>[2x]SNIEV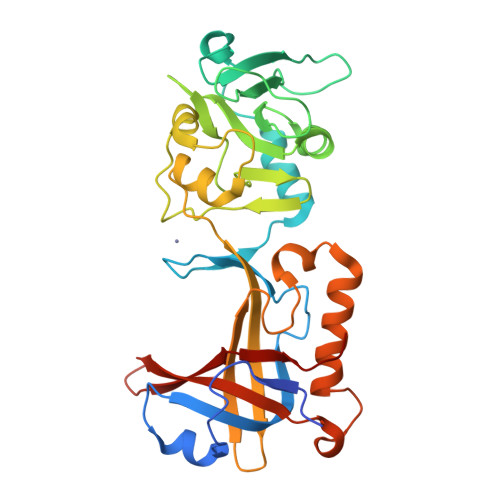ERCQQLSATILTDHQYLERTPLCAILKQKAPQQYRIRAKLRSYKPRRLFQSVKLHCPKCHLLQEVPHEGDLDIIFQDGATKTPDVKLQNTSLYDSKIWTTKNQKGRKVAVHFVKNNGILPLSNECLLLIEGGTLSEICKLSNKFNSVIPVRSGHEDLELLDLSAPFLIQGTIHHYGCKQCSSLRSIQNLNSLVDKTSWIPSSVAEALGIVPLQYVFVMTFTLDDGTGVLEAYLMDSDKFFQIPASEVLMDDDLQKSVDMIMDMFCPPGIKIDAYPWLECFIKSYNVTNGTDNQICYQIFDTTVAEDVI>[2x]MMTGTIETTGNISAEKGGSIILQCHLSSTTAQVTQVNWEQQDQLLAISNADLGWHISPSFKDRVAPGPGLGLTLQSLTVNDTGEYFCIYHTYPDGTYTGRIFLEVLE;>QDVRVQVLPEVRGQLGGTVELPCHLLPPVPGLYISLVTWQRPDAPANHQNVAAFHPKMGPSFPSPKPGSERLSFVSAKQSTGQDTEAELQD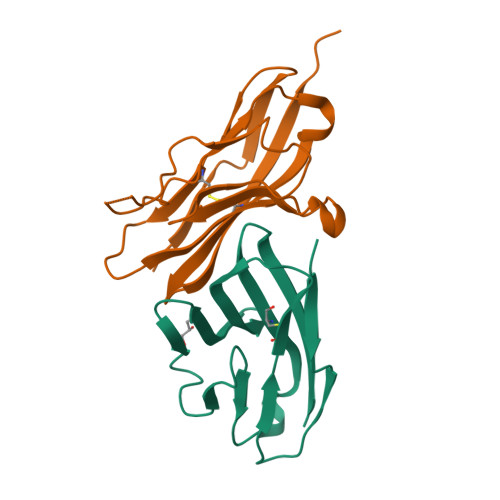ATLALHGLTVEDEGNYTCEFATFPKGSVRGMTWLRVLVPRGSGHHHHHH[2x]>[2x]MGSSHHHHHHSSGLMDSLLGCGVSAAAREPVPRYLTSQPRVSEVAMQSAPLEQPAKRPRCDGSPRTPPSTPPATANLSADDDFQNTDLRTWEPEDVCSFLENRGFREKKVLDIFRDNKIAGSFLPFLDEDRLEDLGVSSLEERKKMIECIQQLSQSRIDLMKVFNDPIHGHIEFHPLLIRIIDTPQFQRLRYIKQLGGGYYVFPGASHNRFEHSLGVGYLAGCLVRALAEKQPELQISERDILCVQIAGLCHDLGHGPFSHMFDGRFIPRARPEKKWKHEQGSIEMFEHLVNSNELKLVMKNYGLVPEEDITFIKEQIMGPPITPVKDSLWPYKGRPATKSFLYEIVSNKRNGIDVDKWDYFARDCHHLGIQNNFDYKRFIKFARICEVEYKVKEDKTYIRKVKHICSREKEVGNLYDMFHTRNCLHRRAYQHKISNLIDIMITDAFLKADPYVEITGTAGKKFRISTAIDDMEAFTKLTDNIFLEVLHSTDPQLSEAQSILRNIECRNLYKYLGETQPKREKIRKEEYERLPQEVAKAKPEKAPDVELKAEDFIVDVINVDYGMEDKNPIDRVHFYCKSNSKQAVRINKEQVSQLLPEKFAEQLIRVYCKKKDGKSLDAAGKHFVQWCALRDFTKPQDGDIIAPLITPLKWNNKTSSCLQEVSKVKTCLKF

The sterile alpha-motif (SAM) and histidine-aspartate (HD) domain-containing protein 1 (SAMHD1) is a dNTP phosphohydrolase that restricts viral replication by limiting the cellular dNTP pool. The active tetramer form of SAMHD1 is induced by cellular nucleotides, which bind two allosteric sites of each subunit. The SAM domain is not required for dNTP hydrolysis and viral restriction by hSAMHD1, but is essential for these activities of mSAMHD1. To better understand the regulatory role of the SAM domain, we crystallized full-length mSAMHD1 in three different states (0, 1, and 2 allosteric nucleotides bound).

In addition to the 2-Allo structure, we also captured crystal structures of full-length mSAMHD1 in two more activation intermediate states: no allosteric nucleotides bound (No-Allo) and one allosteric nucleotide bound to Allo-site 1 only (1-Allo). The 1-Allo crystal was crystallized with dGTP-α-S in the crystallization mixture and diffracted to 3.4 Å resolution. The No-Allo and 1-Allo mSAMHD1 structures also crystallized as tetramers in different space groups (C2 and P21212) with 4 or 2 copies of mSAMHD1 in the asymmetric unit, respectively. However, this symmetry is broken in the 1-Allo tetramer, which is a dimer of dimers, with only one overall twofold axis. Our No-Allo and 1-Allo structures show that these inactive tetramer intermediates are composed of two relatively rigid dimers with loose tetramer interfaces. Although mSAMHD1 is capable of forming tetramers without nucleotides bound to Allo-site 2, these states are inactive and likely represent activation intermediates of the enzyme. Nucleotide binding to Allo-site 1 causes the dimer components to swing around a pivot point and close in toward each other. Starting from the most open No-Allo state, dimer A′ swings progressively toward dimer A via the 1-Allo-state to close the tetramer interface in the 2-Allo state. Since our experiment did not include GTP or dGTP, which are the only allosteric activators to bind Allo-site 115–17, we conclude that some populations of mSAMHD1 protein were purified with GTP or dGTP bound to the allosteric site 1, consistent with the previous observations. These tetramers likely represent activation intermediates similar to our 1-Allo structure, and they are not fully active states of the enzyme.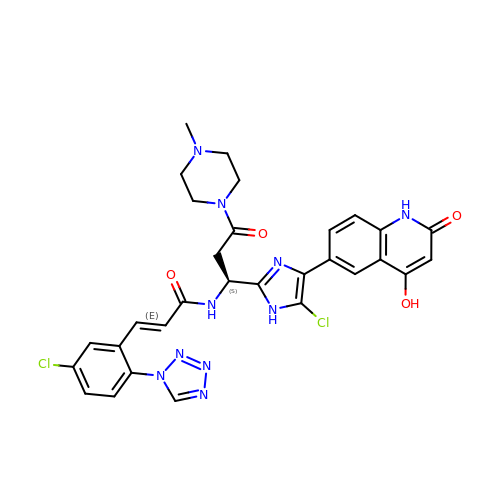(2E)-N-[(1S)-1-[5-chloro-4-(4-hydroxy-2-oxo-1,2-dihydroquinolin-6-yl)-1H-imidazol-2-yl]-3-(4-methylpiperazin-1-yl)-3-oxopropyl]-3-[5-chloro-2-(1H-tetrazol-1-yl)phenyl]prop-2-enamide | C30 H28 Cl2 N10 O4 | NBMJTOOHXJGJNZ-RJOTYRNVSA-N> MARIRDVQGDITEFQGDAIVNAANNYLKLGAGVAGAILRKGGPSIQEECDRIGKIRVGEAAVTG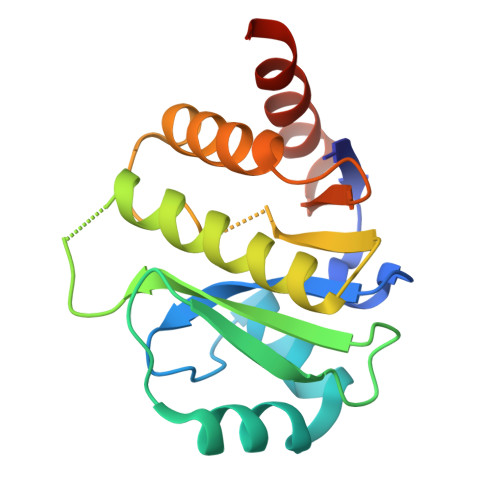AGNLPVRYVIHAAVLGDEPASLETVRKATKSALEKAVELGLKTVAFTALGAWVGGLPAEAVLRVMLEEIKKAPDTLEVTGVHGTEKSAEAARRARLEHHHHHH> MSHHHHHHSMSAAPDSPSSALAALPKDVPNSQPEMVEAVKKHILNMLHLKKRPDVTQPVPKAALLNAIRKLHVGKVGENGYVEIEDDIGRRAEMNELMEQTSEIITFAESGTARKTLHFEISKEGSDLSVVERAEVWLFLKVPKANRTRTKVTIRLFQQQKHPQGSLDTGEEAEEVGLKGERSELLLSEKVVDARKSTWHVFPVSSSIQRLLDQGKSSLDVRIACEQCQESGASLVLLGEEKEQSHRPFLMLQARQSEDHPHRRRRRGLECDGKVNICCKKQFFVSFKDIGWNDWIIAPSGYHANYCEGECPSHIAGTSGSSLSFHSTVINHYRMRGHSPFANLKSCCVPTKLRPMSMLYYDDGQNIIKKDIQNMIVEECGCS

Activins, members of transforming growth factor β (TGF-β) superfamily, were first isolated from porcine ovarian follicular fluid and identified as activating factors for the release of follicle stimulating hormone. Activins function both in autocrine and paracrine manner. They conduce signalling by binding to extracellular domains of type I and type II receptors and allowing the kinase domains of type II receptors to phosphorylate those of type I receptors and initiate the intracellular signalling. Activins, like all other members in the TGF-β superfamily, are synthesized as larger precursors. During the secretory pathway, the precursors are processed by furin-like proteases that cleave the polypeptide after a dibasic recognition sequence between the pro- and mature domains, releasing the mature signalling domain from the covalent linkage to the pro-domain12.

We have engineered the protein to enable proteolytic activation in vitro, by replacing the original furin cleavage site with a HRV 3C protease site and removed two N-terminal cysteine residues, which by analogy to pro-TGF-β1 are likely to interact with the ECM, to avoid interference with native disulfide structure of the rest of the protein. To improve the quality of the crystals, we removed residues 259–282 (reported to be part of heparan sulfate-binding site19) from the pro-domain. The resulting protein yielded significantly better diffracting crystals, enabling us to determine its structure using multi-wavelength anomalous dispersion phasing with selenomethionine-labelled protein. We solved the structure of pro-activin A precursor at 3 Å and refinement of this structure against higher resolution native data yielded a final structure at 2.3 Å. The structure of the pro-activin A precursor consists of two subunit chains that are disulfide-linked at the mature domains. In each subunit, the N terminus of the pro-domain, starting from the first visible residue Q51, forms a helical ‘forearm' region consisting of three α-helices (α1, α2 and α3), a latency lasso and a β-hairpin. In the structure of pro-activin A, two precursor chains form a cross-armed, domain-swapped dimer. Although the electron density for the linker between the pro-domain and the mature domain (Glu301-Arg310) is not visible, it has been confirmed to be intact by SDS–PAGE analysis of dissolved crystals. Size-exclusion chromatography in combination with multiple-angle light scattering (SEC-MALS) analysis shows that pro-activin A is a single species with the expected molecular weight (91.5 kDa, calculated molecular weight 90.9 kDa). This uncleaved pro-activin A precursor is unable to induce the expression of an activin-inducible luciferase reporter gene in HEK293T cells, in agreement with previous findings that cleavage is required for bioactivity.> MDDLKLPRQRVDLVAPPFVHVHEQATKQGPKIMEFKLVVQEKKMVIDEKGTTFQAMTFNGSMPGPLMVVHEGDYVEVTLVNPATNTMPHNIDFHSATGAL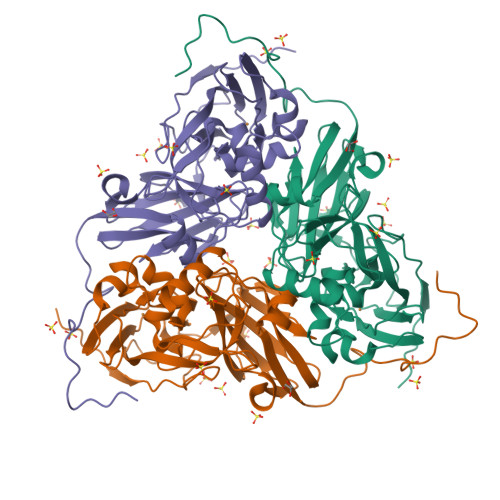GGGALTLINPGEQVVLRWKATRTGVFVYHCAPGGPMIPWHVVSGMNGAVMVLPRDGLNDGHGHSLRYDRIYYIGEQDLYVPRDEKGNFKSYDSPGEAYSDTEEVMRKLTPTHVVFNGKAGALTGKNALNANVGENVLIVHSQANRDSRPHLIGGHGDYVWETGKFSNAPETGLETWFIRGGSAGAALYKFLQPGIYAYVTHNLIEAANLGATAHFKVEGKWNDDLMTQVKAPADIPTGSTNENLYFQGGS> KRNYILGLAIGITSVGYGIIDYETRDVIDAGVRLFKEANVENNEGRRSKRGARRLKRRRRHRIQRVKKLLFDYNLLTDHSELSGINPYEARVKGLSQKLSEEEFSAALLHLAKRRGVHNVNEVEEDTGNELSTKEQISRNSKALEEKYVAELQLERLKKDGEVRGSINRFKTSDYVKEAKQLLKVQKAYHQLDQSFIDTYIDLLETRRTYYEGPGEGSPFGWKDIKEWYEMLMGHCTYFPEELRSVKYAYNADLYNALNDLNNLVITRDENEKLEYYEKFQIIENVFKQKKKPTLKQIAKEILVNEEDIKGYRVTSTGKPEFTNLKVYHDIKDITARKEIIENAELLDQIAKILTIYQSSEDIQEELTNLNSELTQEEIEQISNLKGYTGTHNLSLKAINLILDELWHTNDNQIAIFNRLKLVPKKVDLSQQKEIPTTLVDDFILSPVVKRSFIQSIKVINAIIKKYGLPNDIIIELAREKNSKDAQKMINEMQKRNRQTNERIEEIIRTTGKENAKYLIEKIKLHDMQEGKCLYSLEAIPLEDLLNNPFNYEVDHIIPRSVSFDNSFNNKVLVKQEEASKKGNRTPFQYLSSSDSKISYETFKKHILNLAKGKGRISKTKKEYLLEERDINRFSVQKDFINRNLVDTRYATRGLMNLLRSYFRVNNLDVKVKSINGGFTSFLRRKWKFKKERNKGYKHHAEDALIIANADFIFKEWKKLDKAKKVMENQMFEEKQAESMPEIETEQEYKEIFITPHQIKHIKDFKDYKYSHRVDKKPNRELINDTLYSTRKDDKGNTLIVNNLNGLYDKDNDKLKKLINKSPEKLLMYHHDPQTYQKLKLIMEQYGDEKNPLYKYYEETGNYLTKYSKKDNGPVIKKIKYY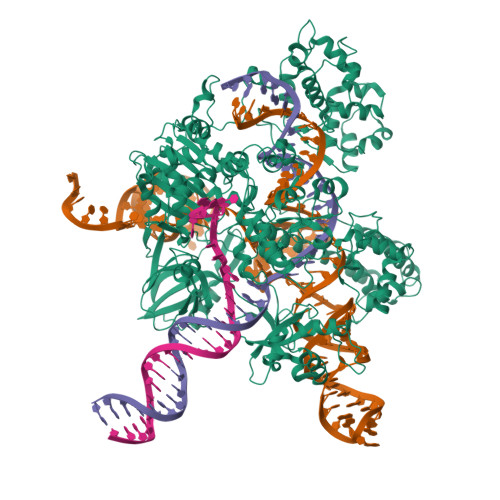GNKLNAHLDITDDYPNSRNKVVKLSLKPYRFDVYLDNGVYKFVTVKNLDVIKKENYYEVNSKCYEEAKKLKKISNQAEFIASFYNNDLIKINGELYRVIGVNNDLLNRIEVNMIDITYREYLENMNDKRPPRIIKTIASKTQSIKKYSTDILGNLYEVKSKKHPQIIKKG RM enzymes prevent the integration, replication and expression of foreign DNA in the host bacterium by introducing double-strand (ds) DNA breaks into the invading genomes. In case of Type ISP enzymes, the entire gamut of tasks is carried out by the coordinated action of target recognition, methyltransferase (MTase), helicase-like ATPase and nuclease domains that constitute the single polypeptide chain. LlaGI recognizes 5′-CTnGAyG-3′, while LlaBIII recognizes 5′-TnAGCC-3′. Like LlaBIII, LlaGI contained six structural domains: the N-terminal Mrr-family nuclease, followed by the N-core and C-core RecA folds of the SF2 helicase-like ATPase domain, connected to the γ-class of N6-adenine MTase domain and the C-terminal TRD by an all α-helical coupler domain.

In continuation of our study of the mechanism of action Type ISP enzymes, we report here the co-crystal structures of a nuclease mutant of LlaGI and a nuclease-deleted mutant LlaGIΔN, bound to DNA substrate mimics. We chose to delete the residues 2–165, producing the recombinant protein LlaGIΔN. The translocation-active nuclease deletion mutant of LlaGI reported here highlights the modular nature of these enzymes. The structures of LlaGIΔN bound to a 22-bp DNA and full-length LlaGI bound to a 28-bp DNA were determined to a resolution of 2.84 and 7.4 Å, respectively. In the LlaGIΔN-DNA crystals there were two molecules in the asymmetric unit, while in LlaGI-DNA there were four. Like in the case of the LlaBIII-DNA complex, in both LlaGI-DNA and LlaGIΔN-DNA structures, the MTase domain and TRD held the target in a vice-like grip. In LlaGIΔN-DNA, the upstream end of the oligonucleotide was not long enough to interact with the ATPase domain. Instead, this end interacted with the ATPase domain of the neighbouring molecule of the asymmetric unit. In the LlaGIΔN structure, only a part of the C-core of chain B could be built with confidence, while the C-core of chain A could not be built due to poor electron density. In the LlaGIΔN and LlaBIII structures, specificity of the T:A base pair is ensured by the interactions made by the flipped adenine with the active site residues of the MTase domain located primarily on Loop I, which catalyse the transfer of methyl group.

>[2x]MRPENVVVKKPKKLRDYQQTAKENALAHFKENDRGQLIMAPGTGKTFTSLKISEALSKDKNGPFKVLYLVPSIQLLTQTLRGWNNDTELTITSMAVTSDRDASRGTDGTEDIKASDIGYPATTSSKKILQNWHDFESLPKQTDMLVVFSTYQSIEVIGEAQKEGFPEFDFIISDEAHRTTGAHEAAKEASAFSKVHSNNNVKGLKRMYQTATPKIYGESAKKNAKDKSILLSSMDDESKYGEVFFRMGFGQAVSRDILTDYKVMVLAVDEAAIQKDMQRTLADPENGLNIDDVGRIVGIWNGMMRRNGYKNPIKNSPYDGAPLERAIAFTRTIEESKKVSSQFEEVVNEYISEAIEDESIHLSMRHADGKMNALQKGEILDWLADPNKPADEARIVSNVRFLTEGIDIPTLDAVIFLSPKKSQVDIVQAVGRIMRKAEGKDYGYIILPIVIPTGEKPETILDNNKNYETVWQVINALRSVDERFEAMIDKLNMAKPKQLKVIGVGSAPEQVNDQDKTIENTPVQTELELEWNKFEGAIFGKIVQKVGDRKYLENWSKDVAKIAERQINWIKNKLSDKKDPISLEFKKFVSSLQHNINDSIDEKQAAEMLSQHLITKPIFEALFSEYSFVNQNPVSQAMESIVSELEKAGFAKEQENLEPLYESVRMRAEGIEKAEDKQKIIVTLYDKFFKTAFKATTERLGIVFTPIEVVDFIVHSVDDVLKKHFGKSLASKDVHILDPFTGTGTFIVRTLTYLKEQMDAGEISLSDITRKFMKELHANEIVLLSYYIAAINIEATFDEINGEEEGYVPFEGIVLTDTFESTETEETLDDDYFGTNDERLKRQQEVPITAIIGNPPYSKGQSNENDNNKNIEYPRLFKSIADSYVKNSKTTSVLGMYDSYVLSIRWASNRLNDKGVIGFVSNGSYIDSQSADGLRKSLFKEFNHLYIFNLRGDQRTQGETSRKEGGKIFGSGSRTSIAISILVKDDSDNHEVHYHDIGDYLTRDDKLDILRDKESILNIDWENISPDENNDWINQRDQNYLNYRPLADENGSIFSVKDIGIVTNRDAWVSNFSKINVSDNVQIMIKNYNLEVDRLENIDVKLNDKTVVDYVTNDERKISWSRSLKQRAARREKTQFSHSDIMLAMYRPFTKKYLYRNRFLNENVRKTYQTFPDKNSKNLLINISGQGDKADFATLISEYLSDMHVIGGQARNLPRFTYETDGMFAGRTDNIVSDDEFYYVYGVLHSSAYRKRYANDLKKDLPRIPLLKNKDKYVEIGRKLSDLHLNYENQPIWDGIEVEISQPDYRVKKMKHPKKGVLDTIIYNESITIKNIPERAYEYVVNGRPAIEWIIDQYQVKTDKKSGITDDPNEFSDNPKYILNLLLSVITVSMRTLELIEELPEFEIQE> DDDLVDAEGNLVENGGTYYLLPHIWAHGGGIETAKTG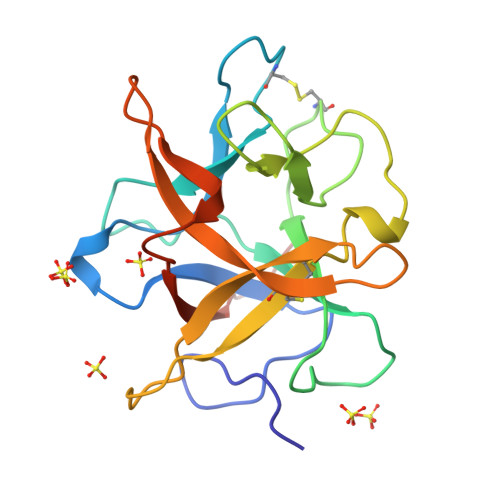NEPCPLTVVRSPNEVSKGEPIRISSQFLSLFIPRGSLVALGFANPPSCAASPWWTVVDSPQGPAVKLSQQKLPEKDILVFKFEKVSHSNIHVYKLLYCQHDEEDVKCDQYIGIHRDRNGNRRLVVTEENPLELVLLKAKSETASSH> MFRQSLLRLPWWNFQTEHRQRCVMMYGGARTKNTHNANHRVYVRKFKRNAFPNRTRHHWAVSMTGVQG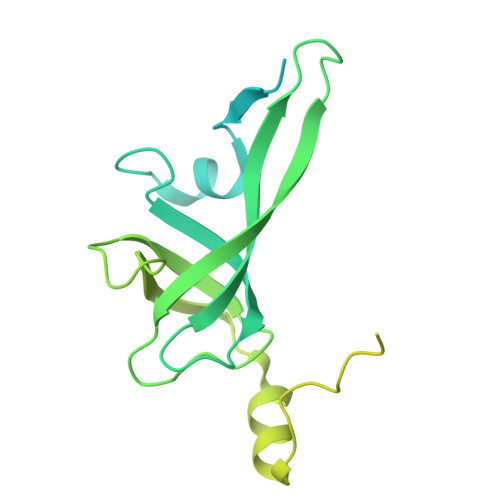QRPRRMPWPYDLTSMIFNQPRQGSDKIGYVVGTSMLKTAVVAANHMVYYPKFNQRVSRTSRFFAHDEDLACVEGDLVHIKQSRKISKYKHYYVFSILEPNIEGRERLKLGLKAVPPPLFGYPVSRRVVKLNLTNTEGTKEKLAAAIQEHVQDAYRFAGPTPDQPRAKLTDSASFDEANKMIAPNSSVTAELPPGAEPAFLGDGQPVAEEFSEVEEDSRHKKGDDYWMNLQPSDKYDFKNLKKSP>XMEIDKELAPQDRTVTVATVLPAVPGPSPLTIKQPFQSEVLFAGTKDAEASLTIANIDSVSTLTTFYRHASLESLWVTIHPTLQAPTFPTTVGVCWVPAQSPVTPAQITKTYGGQIFCIGGAIQTLSPLIVKCPLEMMQPRVKDSIQ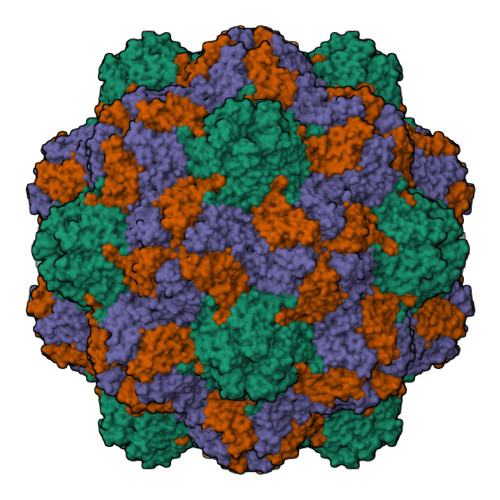YLDSPKLLISITAQPTAPPASTCIITVSGTLSMHSPLITDTST[3x]> SNAQIDGFVRTLRARPEAGGKVPVFVFHPAGGSTVVYEPLLGRLPADTPMYGFERVEGSIEERAQQYVPKLIEMQGDGPYVLVGWSLGGVLAYACAIGLRRLGKDVRFVGLIDAVRAGEEIPQTKEEIRKRWDRYAAFAEKTFNVTIPAIPYEQLEELDDEGQVRFVLDAVSQSGVQIPAGIIEHQRTSYLDNRAIDTAQIQPYDGHVTLYMADRYHDDAIMFEPRYAVRQPDGGWGEYVSDLEVVPIGGEHIQAIDEPIIAKVGEHMSRALGQIEADRTSEVGKQ

Pks13 is a multidomain enzyme that performs the final step in the synthesis of mycolic acids through the condensation of a long-chain fatty acid (C24–C26) and a very long-chain fatty acid (C56).12 The product is transferred from Pks13 to trehalose by the Pks13-TE domain. Pks13 fulfills a critical function for Mtb by performing a condensation reaction of a long-chain fatty acid and a very long-chain meromycolic acid to form a mycolic acid. Pks13-TE is a validated target for the development of antibiotics for Mtb. In previous work, we identified TAM16, a potent lead molecule for Pks13-TE. X-ray crystallography verified that compounds from all three different series were binding deep within the active site of Pks13-TE, displacing the side chain of Arg1563 with atoms within about 4 Å from the catalytic Ser1533 OG.

The structure of the series 2 compound X20419 in complex with Pks13-TE was solved using X-ray diffraction data collected to 2.2 Å resolution. Crystals were in the tetragonal P41212 space group with one molecule per asymmetric unit. X20419 was found to reside within the same channel as that for X20404, extending through the core of Pks13-TE via a conformational change in the Arg1563 side chain. Most of the contacts between the protein and the inhibitor are VDW/hydrophobic interactions with the addition of two hydrogen bonds: between the N9 of the indole ring of R1 and the carbonyl of Ala1561, at 3.3 Å, and a weak bond between the catalytic Ser1533 OG to the carbonyl (O21) of the inhibitor, at 3.2 Å. The terminal aromatic ring system of R1 forms VDW interactions with the carbons of the Arg1563 side chain. Two methoxy substituents on the ring contact the Ile1648, Ile1643, and Tyr1686 side chains. The piperidine ring of R1 is angled to achieve a pi-stacking interaction between the pyrimidine ring and Phe1670. The piperidine overlaps with the position of the piperidine in the TAM16-bound structure, while the pyrimidine extends into a space occupied by the benzofuran of TAM16, without causing the Phe1670 side chain flip. The enamine linker of R2 places the terminal phenyl into a hydrophobic pocket created by the side chains of the Phe1670, Tyr1637, Arg1572, Arg1641, and Trp1579. The C16 of the piperidine is also 3.4 Å away from the catalytic Ser1533 OG, in addition to the H-bond to O21, thoroughly blocking substrate access.> ANPCCSNPCQNRGECMSTGFDQYKCDCTRTGFYGEN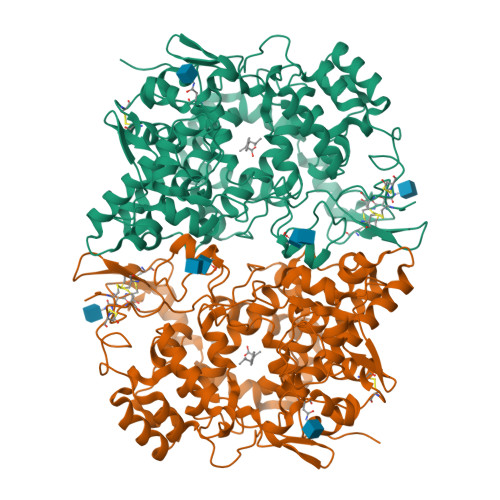CTTPEFLTRIKLLLKPTPNTVWYILTHFKGVWNIVNNIPFLRSLIMKYVLTSRSYLIDSPPTYNVHYGYKSWEAFSNLSYYTRALPPVADDCPTPMGVKGNKELPDSKEVLEKVLLRREFIPDPQGSNMMFAFFAQHFTHQFFKTDHKRGPGFTRGLGHGVDLNHIYGETLDRQHKLRLFKDGKLKYQVIGGEVYPPTVKDTQVEMIYPPHIPENLQFAVGQEVFGLVPGLMMYATIWLREHNRVCDILKQEHPEWGDEQLFQTSRLILIGETIKIVIEDYVQHLSGYHFKLKFDPELLFNQQFQYQNRIASEFNTLYHWHPLLPDTFNIEDQEYSFKQFLYNNSILLEHGLTQFVESFTRQIAGRVAGGRNVPIAVQAVAKASIDQSREMKYQSLNEYRKRFSLKPYTSFEELTGEKEMAAELKALYSDIDVMELYPALLVEKPRPDAIFGETMVELGAPFSLKGLMGNPICSPQYWKPSTFGGEVGFKIINTASIQSLICNNVKGCPFTSFNVQDPQPTKTATINASASHSRLDDINPTVLIKRRSTEL(3S,7S,11E)-7,14,16-trihydroxy-3-methyl-3,4,5,6,7,8,9,10-octahydro-1H-2-benzoxacyclotetradecin-1-one 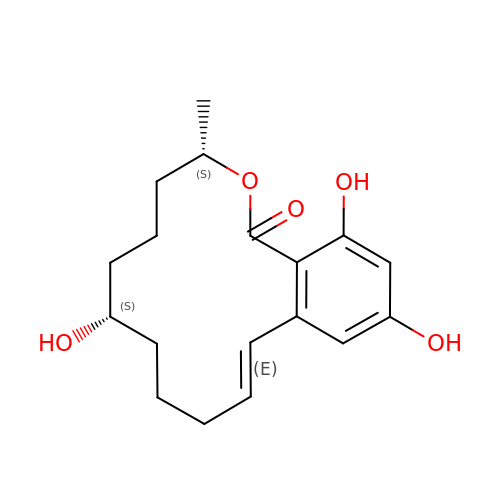| C18 H24 O5 | FPQFYIAXQDXNOR-PMRAARRBSA-N>WVQPITCQKPSLTLWLDDKMFTGLINTGADVTIIKLEDW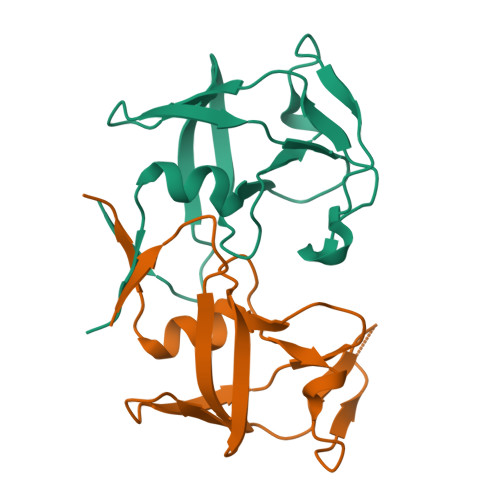PPNWPITDTLTNLRGIGQSNNPKQSSKYLTWRDKENNSGLIKPFVIPNLPVNLWGRDLLSQMKIMMCSPNDIVTA[2x]> GDELYRQSLEIISRYLREQATGAKDTKPMGRSGATSRKALETLRRVGDGVQRN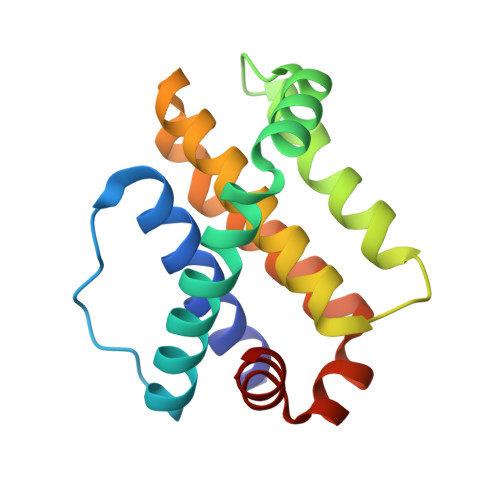HETAFQGMLRKLDIKNEDDVKSLSRVMIHVFSDGVTNWGRIVTLISFGAFVAKHLKTINQESCIEPLAESITDVLVRTKRDWLVKQRGWDGFVEFFH>[2x]MFYKEENFKKTEIGEIPEDWEIVELKDVCKKIKAGGTPKTSVEEYYKNGTIPFVKIEDITNSNKYLTNTKIKITEEGLNNSNAWIVPKNSVLFAMYGSIGETAINKIEVATNQAILGIIPKDNILESEFLYYILAKNKNYYSKLGMQTTQKNLNAQIVKSFKI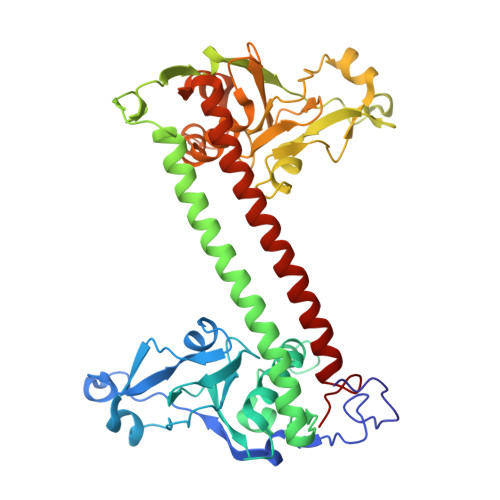PLPPLEEQKQIAKILTKIDEGIEIIEKSINKLERIKKGLMHKLLTKGIGHSRFKKSEIGEIPEDWEVFEIKDIFEVKTGTTPSTKKSEYWENGEINWITPLDLSRLNEKIYIGSSERKVTKIALEKCNLNLIPKGSIIISTRAPVGYVAVLTVESTFNQGCKGLFQKNNDSVNTEFYAYYLKFKKNLLENLSGGSTFKELSKSMLENFKIPLPPLEEQKQIAKILSSVDKSIELKKQKKEKLQRMKKKIMELLLTGKVRVKT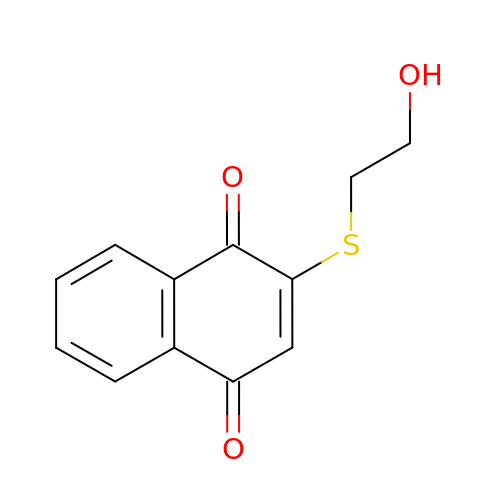2-[(2-hydroxyethyl)sulfanyl]naphthalene-1,4-dione | C12 H10 O3 S | IBLOZMPODBITIK-UHFFFAOYSA-N>MAHHHHHHMPKKSMHATRNDLPSNTKTTMIALLNENLAATIDLALITKQAHWNLKGPQFIAVHEMLDGFRAELDDHVDTIAERAVQIGGTAYGTTQVVVKESRLKPYPTDIYAVHDHLVALIER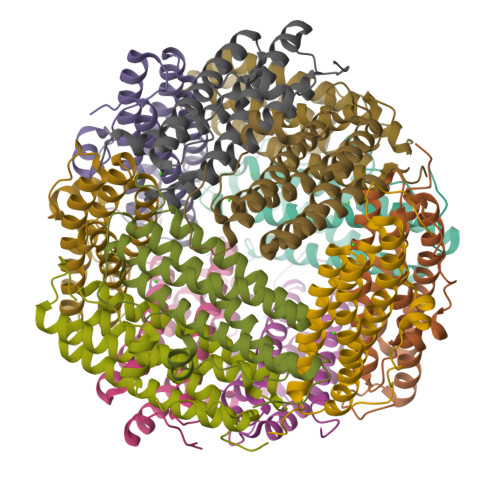YGDVANLVRKSIKDADDAGDDDTADIFTAASRSLDKALWFLEAHVQESN[12x]> APAVADKADNAFMMICTALVLFMTIPGIAL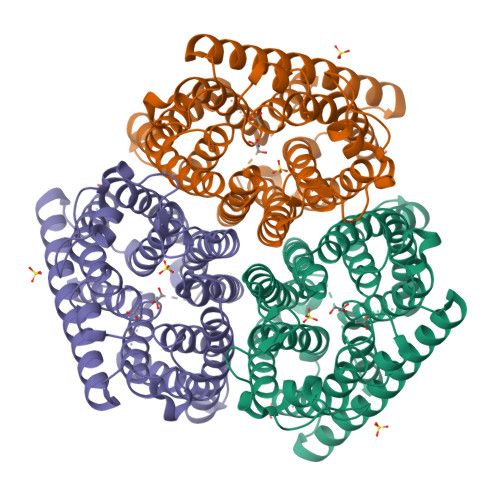FYGGLIRGKNVLSMLTQVTVTFALVCILWVVYGYSLAFGEGNNFFGNINWLMLKNIELTAVMGSIYQYIHVAFQGSFACITVGLIVGALAERIRFSAVLIFVVVWLTLSYIPIAHMVWGGGLLASHGALDFAGGTVVHINAAIAGLVGAYLIGKRVGFGKEAFKPHNLPMVFTGTAILYIGWFGFNAGSAGTANEIAALAFVNTVVATAAAILGWIFGEWALRGKPSLLGACSGAIAGLVGVTPACGYIGVGGALIIGVVAGLAGLWGVTMLKRLLRVDDPCDVFGVFGVCGIVGCIMTGIFAASSLGGVGFAEGVTMGHQLLVQLESIAITIVWSGVVAFIGYKLADLTVGLRVPEEQEREGLDVNSHGENAYNADQAQQPAQADLEHHHHHH>[4x]MSLNLTIGTSKFNPPFEVWSGNNSSLYGFDIDLMQEICRRLH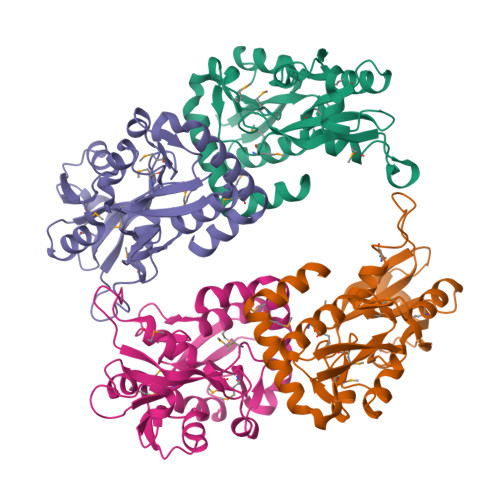ATCTFEAYIFDDLFPALKNREVDLVIASMIITDERKKHFIFSLPYMESNSQYITTVDSKISTFDDLHGKKIGVRKGTPYARQVLSENRNNQVIFYELIQDMLLGLSNNQVDASLMDYEAAKYWMASEPYAYKLIGKKYKLIGKKISIGEGYSIMANPDQFVLIKKINKILLEMEADGTYLRLYSEYFEGHHHHHH>MGKFGFFDDANKEYVITVPRTPYPWINYLGTENFFSLISNTAGGYSFYRDARLRRITRYRYNNVPIDMGGRYFYIYDNGDFWSPGWSPVKRELESYESRHGLGYTKIAGKRNGIKAEVTFFVPLNYNGEVQKLILKNEGQDKKKITLFSFIEFSLWNAYDDMTNFQRNFSTGEVEIEGSVIYHKTEYRERRNHYAFYSVNAKISGFDSDRDSFIGLYNGFDAPQAVVNGKSNNSVADGWAPIASHSIEIELNPGEQKEYVFIIGYVENKDEEKWESKGVINKKKAYEMIEQFNTVEKVDKAFEELKSYWNALLSKYFLESHDEKLNRMVNIWNQYQSMVTFNMSRSASYFESGIGRGMGFRDSNQDLLGFVHQIPERARERLLDLAATQLEDGSAYHQYQPLTKKGNNEIGSNFNDDPLWLILATAAYIKETGDYSILKEQVPFNNDPSKADTMFEHLTRSFYHVVNNLGPHGLPLIGRADWNDCLNLNCFSTVPDESFQTTTSKDGKVAESVMIAGMFVFIGKDYVKLSEYMGLEEEARKAQQHIDAMKEAILKYGYDGEWFLRAYDDFGRKVGSKENEEGKIFIESQGF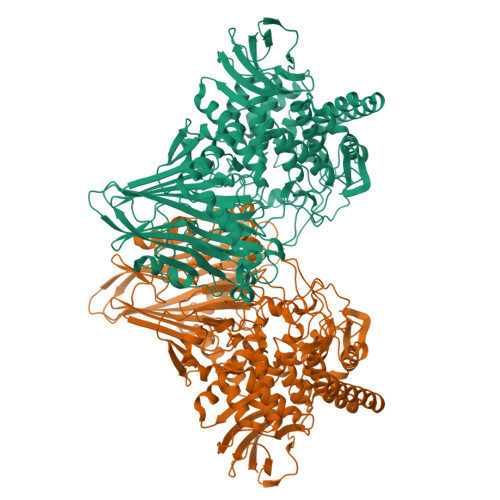SVMAEIGLEDGKALKALDSVKKYLDTPYGLVLQNPAFTRYYIEYGEISTYPPGYKENAGIFSHNNAWIISAETVVGRGDMAFDYYRKIAPAYIEDVSDIHKLEPYVYAQMVAGKDAKRHGEAKNSWLTGTAAWNFVAISQWILGVKPDYDGLKIDPSIPKAWDGYKVTRYFRGSTYEITVKNPNHVSKGVAKITVDGNEISGNILPVFNDGKTHKVEVIMGLEHHHHHH[2x]[2-(1,3-thiazol-4-yl)-1H-benzimidazol-1-yl]acetic acid | C12 H9 N3 O2 S | 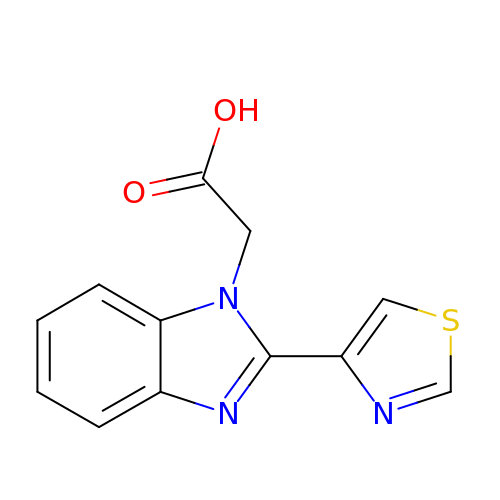QJFKGTPZZBLCJY-UHFFFAOYSA-N>EKDRKRILITGGAGFVGSHLTDKLMMDGHEVTVVDNFFTGRKRNVEHWIGHENFELINHDVVEPLYIEVDQIYHLASPASPPNYMYNPIKTLKTNTIGTLNMLGLAKRVGARLLLASTSEVYGDPEVHPQSEDYWGHVNPIGPRACYDEGKAVAETMCYAYMKQEGVEVRVARIFNTFGPRMHMNDGRVVSNFILQALQGEPLTVYGSGSQTRAFQYVSDLVNGLVALMNSNVSSPVNLGNPEEHTILEFAQLIKNLVGSGSEIQFLSEAQDDPQKRKPDIKKAKLMLGWEPVVPLEEGLN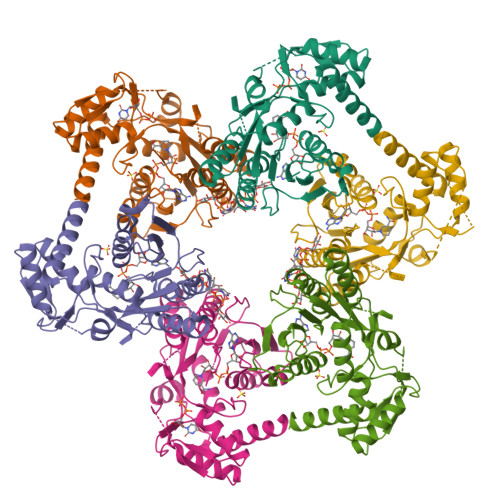KAIHYFRKELEYQANNQYIPKPKPARIKKGRTRHS[6x]>PMKTI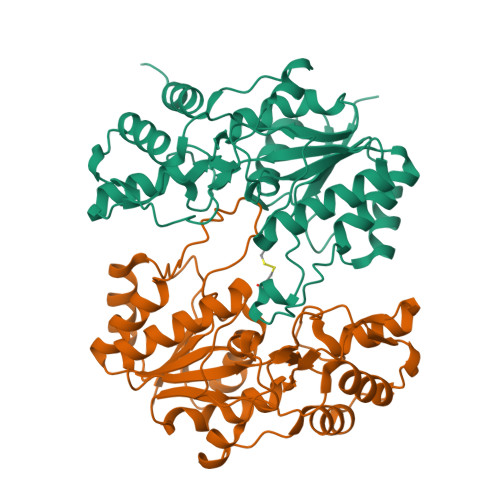LVTGGSGFLGRRLVSHLSKNYTVVAPTHGELDLTDREKIISEVTKINPQIIIHTAAISNTGLCEQNPELSESINLNGTKYLAEAASKINSKLIFCSSDQIYNGNAEKGPLSEDIDVHPVNVYGKHKLEAERKLQEILPTSVSLRLTWMYDHPSSKIPQHKNLPIMLLEAKEKNVPFVTTVNEYRAITFVGEVVENIEKTFELPGGVYNYGASNTSNSYETYKEIAKIMDVPENLVENDTNRFKAQARNISMNIQKIEKHGIHFSNTVDGFSKMYKSFSNSE[4x]>GSAKDPKMPLHILTHRECEVLQLLTDGKSNRGIGETLFISEKTVKNHVSSILQKMKVNDRTQAVVT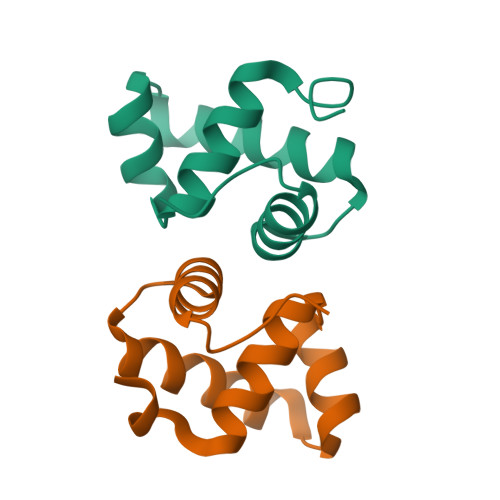AIKHGWVYIR[2x]> SGDYRVQNTSLEAIVQNASSDNQGIQLSAVQAARKLLSSDRNPPIDDLIKSGILPILVHCLERDDNPSLQFEAAWALTNIASGTSEQTQAVVQSNAVPLFLRLLHSPHQNVCEQAVWALGNIIGDGPQCRDYVISLGVVKPLLSFISPSIPITFLRNVTWVMVNLCRHKDPPPPMETIQEILPALCVLIHHTDVNILVDTVWALSYLTDAGNEQIQMVIDSGIVPHLVPLLSHQEVKVQTAALRAVGNIVTGTDEQTQVVLNCDALSHFPALLTHPKEKINKEAVWFLSNITAGNQQQVQAVIDANLVPMIIHLLDKGDFGTQKEAAWAISNLTISGRKDQVAYLIQQNVIPPFCNLLTVKDAQVVQVVLDGLSNILKMAEDEAETIGNLIEECGGLEKIEQLQNHENEDIYKLAYEIIDQFFSSDDIDEDPSLVPEAIQGGTFGFNSSANVPTEGFQF;> SRSLNMLGRKTCLGRRVVQPGMFADYPPTKKARVLLRRMSN

Active transport of proteins from the cytoplasm to the nucleus is mediated by a family of nuclear transport receptors known as importins (or karyopherins), together with a number of ancillary proteins including nucleoporins and Ran1–3. Importin α is constructed from an N-terminal importin β-binding (IBB) domain and a C-terminal NLS binding domain featuring ten armadillo (ARM)-repeat motifs. The W proteins of henipaviruses share a common N-terminal domain with P and V proteins, but have a unique NLS bearing C-terminal domain that is recognised preferentially by importins α3 and α4 (KPNA4 and KPNA3), rather than the better characterised importin α1 (KPNA2). In this study, we present high-resolution structures of importin α isoform adaptors bound to the NLS regions of HeV W and NiV W, providing insights into the molecular basis of importin α isoform specificity.

The structure of the importin α3:HeV W complex was determined in three different space groups, with all crystals exhibiting highly similar structures (r.m.s.d < 0.35) and containing one HeV W NLS chain bound to a single importin α3 chain (the highest resolution structure of 1.6 Å will be used for further discussion and analysis). However, there were marked differences residing outside this region, with importin α3 ARM repeats 6–9 binding HeV W and NiV W residues 419–444 and 421–446, respectively. Notably, despite binding the same region of HeV W and NiV W, importin α3 exhibited a 2.4-fold more extensive interaction buried surface area than importin α1, with 16 additional hydrogen bonds, and six additional salt bridge interactions, consistent with its > 50-fold higher affinity. To gain insights into the basis of isoform specificity, we superimposed the structures of importin α1:HeV W and importin α3:HeV W, and found the structures to be highly similar, with an r.m.s.d. of 1.1 Å across 411 residues, except for the positioning of ARM repeats 7 and 8. Notably, in importin α1, ARM repeats 7 and 8 are positioned closer to the inner surface of the NLS-binding interface, whereas in importin α3, these regions are positioned in a more open conformation. To probe the interaction of the importin α3:HeV W interface in greater detail, we designed mutations to disrupt key salt bridges at the major and minor sites of importin α3. Similarly, mutations predicted to disrupt interaction at the importin α3 major site, K437A/K438A and K437D/K438D in HeV W C-terminal domain, and K439A/K440A and K439D/K440D in the NiV W C-terminal domain, also failed to interact with importin α3. Consistent with these results, we found that mutations in both the major and minor site-binding regions of HeV W disrupted the affinity of interaction to importin α3 in ELISA, and resulted in reduced nuclear accumulation.> MEVVSLPRLGEPAPAFEAQTTFGPVKFPDDFKGQWVVLFSHPADFTPVCTTEFVAFAKNYEEFKKRNVQLIGLSVDSNFSHIAWVMNIKEKFGIEIPFPIIADHNMEVAKKYGMIHPAQSTTFTVRALFVIDDKGILRAMIYYPLTTGRNIREV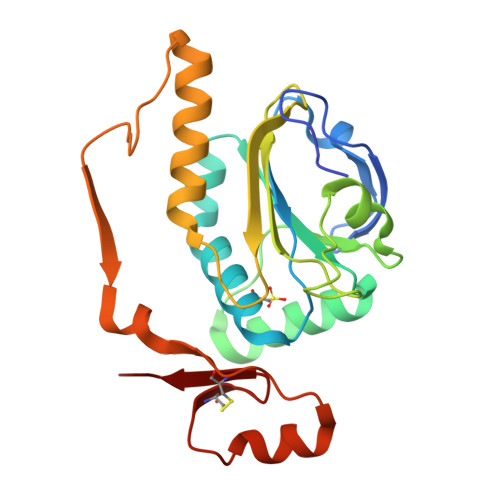IRLVDALQTADREGVATPADWVPEPQTWEFTEENTKVIVPPPTTYEDAVKRLQEGYECADWYICKKKVA> MKKEVRKVRIALASPEKIRSWSYGEVEKP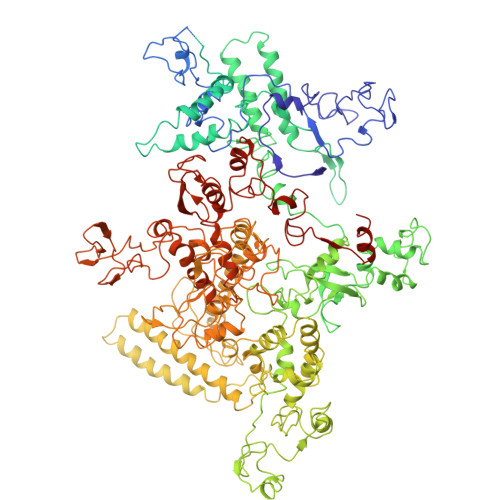ETINYRTLKPERDGLFDERIFGPIKDYECACGKYKRQRFEGKVCERCGVEVTRSIVRRYRMGHIELATPAAHIWFVKDVPSKIGTLLDLSATELEQVLYFNKYIVLDPKGAVLDGVPVEKRQLLTDEEYRELRYGKQETYPLPAGVDALVKDGEEVVKGQELAPGVVSRMDGVALYRFPRRVRVDYLRKERAALRIPLSAWVEKEAYRPGEVLAELSEPYLFRAEESGVVELKDLAEGHLIYLRQEEEVVARYFLPAGMTPLVVEGEIVEVGQPLAEGKGLLRLPRHMTAKEVEAEEEGDSVHLTLFLEWTEPKDYKVAPHMNVIVPEGAKVQAGEKIVAAIDPEEEVIAEAEGVVHLHEPASILVVKARVYPFEDDVEVTTGDRVAPGDVLADGGKVKSEIYGRVEVDLVRNVVRVVESYDIDARMGAEAIQELLKELDLEKLERELLEEMKHPSRARRAKARKRLEVVRAFLDSGNRPEWMILEAVPVLPPDLRPMVQVDGGRFATSDLNDLYRRLINRNNRLKKLLAQGAPEIIIRNEKRMLQEAVDAVIDNGRRGSPVTNPGSERPLRSLTDILSGKQGRFRQNLLGKRVDYSGRSVIVVGPQLKLHQCGLPKRMALELFKPFLLKKMEEKAFAPNVKAARRMLERQRDIKDEVWDALEEVIHGKVVLLNRAPTLHRLGIQAFQPVLVEGQSIQLHPLVCEAFNADFDGDQMAVHVPLSSFAQAEARIQMLSAHNLLSPASGEPLAKPSRDIILGLYYITQVRKEKKGAGMAFATPEEALAAYERGEVALNAPIVVAGRETSVGRLKFVFANPDEALLAVAHGLLDLQDVVTVRYLGRRLETSPGRILFARIVGEAVGDEKVAQELIQMDVPQEKNSLKDLVYQAFLRLGMEKTARLLDALKYYGFTLSTTSGITIGIDDAVIPEEKQRYLEEADRKLRQIEQAYEMGFLTDRERYDQVIQLWTETTEKVTQAVFKNFEENYPFNPLYVMAQSGARGNPQQIRQLCGMRGLMQKPSGETFEVPVRSSFREGLTVLEYFISSHGARKGGADTALRTADSGYLTRKLVDVAHEIVVREADCGTTNYISVPLFQMDEVTRTLRLRKRSDIESGLYGRVLAREVEALGRRLEEGRYLSLEDVHFLIKAAEAGEVREVPVRSPLTCQTRYGVCQKCYGYDLSMARPVSIGEAVGVVAAESIGEPGTQLTMRTFHTGGVAVGTDITQGLPRVIELFEARRPKAKAVISEIDGVVRIEEGEDRLSVFVESEGFSKEYKLPKDARLLVKDGDYVEAGQPLTRGAIDPHQLLEAKGPEAVERYLVDEIQKVYRAQGVKLHDKHIEIVVRQMLKYVEVTDPGDSRLLEGQVLEKWDVEALNERLIAEGKVPVAWKPLLMGVTKSALSTKSWLSAASFQNTTHVLTEAAIAGKKDELIGLKENVILGRLIPAGTGSDFVRFTQVVDQRTLKAIEEARKEAVEAKEKEAPRRPVRREQPGKGL> ANIVGGIAYSINNASLCS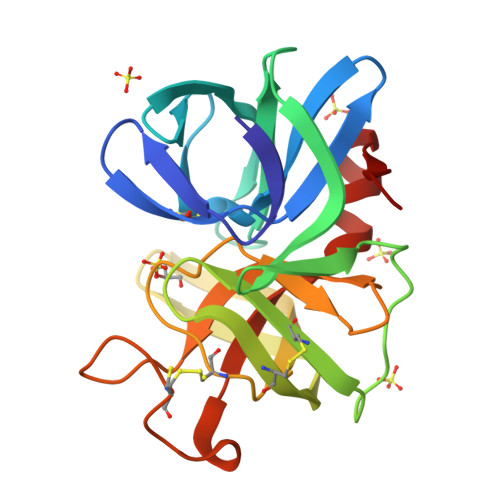VGFSVTRGATKGFVTAGHCGTVNATARIGGAVVGTFAARVFPGNDRAWVSLTSAQTLLPRVANGSSFVTVRGSTEAAVGAAVCRSGSTTGYQCGTITAKNVTANYAEGAVRGLTQGNACMGRGDSGGSWITSAGQAQGVMSGGNVQSNGNNCGIPASQRSSLFERLQPILSQYGLSLVTG> GSQQNKNAPSTAGLGYGSWEIDPKDLTFLKELGTGQFGVVKYGKWRGQYDVAIKMIKEGSMSEDEFIEEAKVMMNLSHEKLVQLYGVCTKQRPIFIITEYMANGCLLNYLREARHAFQTQQLLEMCKDV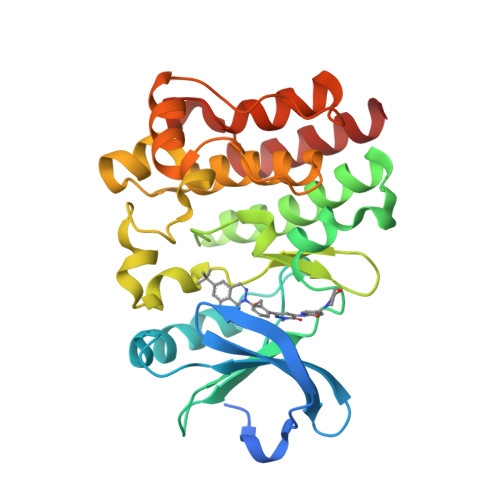CEAMEYLESKQFLHRDLAARNCLVNDQGVVKVSDFGLSRYVLDDEYTSSVGSKFPVRWSPPEVLMYSKFSSKSDIWAFGVLMWEIYSLGKMPYERFTNSETAEHIAQGLRLYRPHLASAAVYTIMYSCWHEKADERPTFKILLSNILDVMDEES>WGLNNAARADGKLWFGTAADIPGLEQDDRYYMKEYNNTHDFGGTTPANIMKFMFTEPEQNVFNFTGAQEFLDIAFASHKLVRCHNLIWQSELPTWVTNPTTNWTNETLSKVLQNHVYTLVSHFGDQCYSWDVVNEALSDDPAGSYQNNIWFDTIGPEYVAMAFEYAEKAVKDHKLNVKLYYNDYNIEYPGPKSTAAQNIVKELKARNIQIDGVGLESHFIAGETPSQATQITNMADFTSLDIDVAVTELDVRLYLPPNATSEAQQVADYYATVAACAATERCIGITVWDFDDTYSWVPSTFAGQGYADLFFQPDGPNTP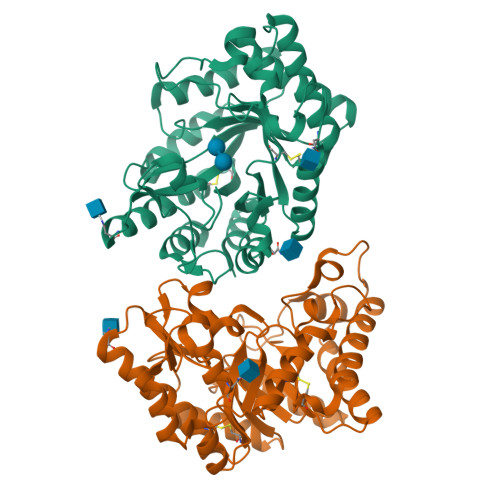LVKKAAYDGCLQALQH[2x]In response to environmental stimuli, the bacterium produces and secretes its main virulence factor, the cholera toxin (CT). CT is an AB5 protein toxin, which consists of one toxic A-subunit (CTA) and five identical B-subunits arranged in a doughnut-shaped ring (CTB). The primary receptor of the cholera toxin is the GM1 ganglioside, which is expressed in distinct membrane microdomains of small-intestinal epithelial cells. There are two major biotypes of V. cholerae, classical and El Tor, which produce cholera toxins with a slight sequence variation (cCT and ET CT). cCT and ET CT differ in only two residues of the B-subunit, His18/Tyr18 and Thr47/Ile47 (classical/El Tor).

Moreover, no previous toxin structure has been reported in complex with the blood group H determinant, which is characteristic of blood group O. The crystal structures of the cCTB and ET CTB complexes were determined to a resolution of 1.1 Å and 1.5 Å, respectively. Both proteins crystallized using the same conditions, but in different space groups (P212121 and P21). Well-defined electron density is present in all ten binding sites of the two pentamers, although the ligand orientations differ. While the electron density of the cCTB structure primarily supports orientation 2, most ET CTB binding sites exhibit the ligand in orientation 1. Since H-tetra-BGA is an almost symmetrical molecule, the fucosyl residues are indistinguishable. As for the complexes with A-penta-BGA, the fucose near residue 47 is most tightly anchored to the toxin, while the other fucose is loosely bound, by indirect water-mediated interactions. In general, the two structures are very similar, except that the N-acetyl group changes place in the two different orientations; the axial 4-OH group of Gal is mimicked by the α-anomer of GlcNAc. In orientation 1, the N-acetyl group takes the position of the GalNAc residue characterizing A-penta-BGA. For one, only the H-determinant, but not the A-determinant, can bind to the toxin in two alternative orientations, likely contributing to its increased affinity.

>[10x]TPQNITDLCAEYHNTQIYTLNDKIFSYTESLAGKREMAIITFKNGAIFQVEVPGSQHIDSQKKAIERMKDTLRIAYLTEAKVEKLCVWNNKTPHAIAAISMAN> MSFIFIPTVRTLHQAELVLNHKNTYLRVNSSHMEVPQLVEFIHQLVDKYPGQKIYVDLQGSKIRISRSQPNLILTKDQSVELTIKAPTKDTKAIHIGNPNTIKLLSQGTHVKIDDGRMEIVVNSIKDSETAIATVIKGGELKPGKGFNLQPHPFVQNQLSERDAEIVEKLKDVKEVCFALSFVCVVEEIQDLKKRSNGKYIVAKIEREMDLERLKAISSQCNEIWICRGDMGVQLGFVGMAKFVREYTTFMKQLNCPSIMAGEVMEHLCDNTIPTRSEICYLGNLIADGYNGIVLSDETVFGKYPQQTMDFCYDFVQQY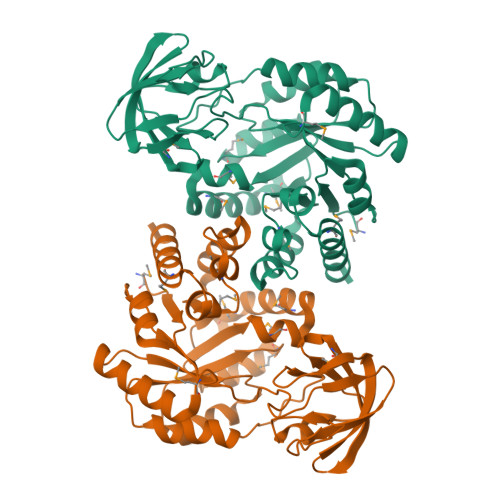LN> GHHHHHHAENLYFQGHMVAIPGGTFRMGGEDPDAFPEDGEGPVRTVRLSPFLIDRYAVSNRQFAAFVKATGYVTDAERYGWSFVFHAHVAPGTPVMDAVVPEAPWWVAVPGAYWKAPEGPGSSITDRPNHPVVHVSWNDAVAYATWAGKRLPTEAEWEMAARGGLDQARYPWGNELTPRGRHRCNIWQGTFPVHDTGEDGYTGTAPVNAFAPNGYGLYN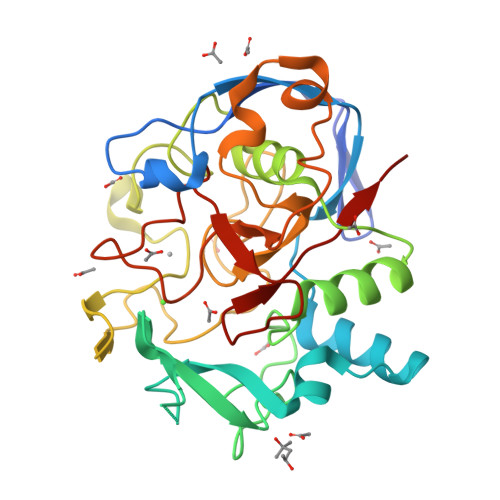VAGNVWEWCADWWSADWHATESPATRIDPRGPETGTARVTKGGSFLCHESYCNRYRVAARTCNTPDSSAAHTGFRCAADPL> SNAAQFKEGEHYQVLKTPASSSPVVSEFFSFYCPHCNTFEPIIAQLKQQLPEGAKFQKNHVSFMGGNMGQAM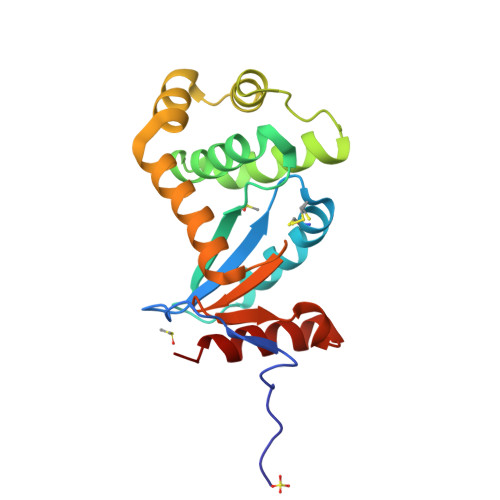SKAYATMIALEVEDKMVPVMFNRIHTLRKPPKDEQELRQIFLDEGIDAAKFDAAYNGFAVDSMVHRFDKQFQDSGLTGVPAVVVNNRYLVQGQSAKSLDEYFDLVNYLLTLK>[4x]MTSVRENILFGMGNPLLDISAVVDKDFLDKYSLKPNDQILAEDKHKELFDELVKKFKVEYHAGGSTQNSIKVAQWMIQQPHKAATFFGCIGIDKFGEILKRKAAEAHVDAHYYEQNEQPTGTCAACITGDNRSLI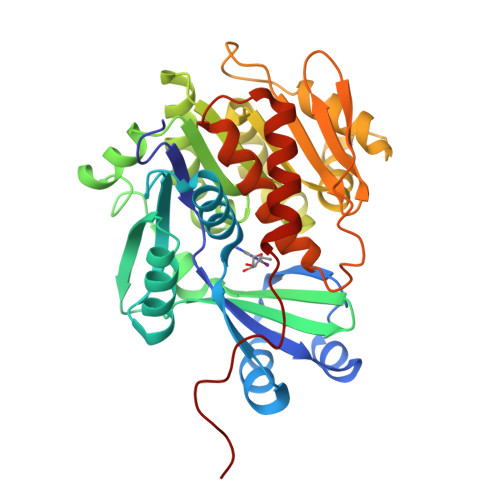ANLAAANCYKKEKHLDLEKNWMLVEKARVCYIAGFFLTVSPESVLKVAHHASENNRIFTLNLSAPFISQFYKESLMKVMPYVDILFGNETEAATFAREQGFETKDIKEIAKKTQALPKMNSKRQRIVIFTQGRDDTIMATESEVTAFAVLDQDQKEIIDTNGAGDAFVGGFLSQLVSDKPLTECIRAGHYAASIIIRRTGCTFPEKPDFH>SNANTYTAEEVVESGHRFFGSTSGGIASAVEKAFQSFGLPNGYILGEEGSGAFIGGLTYGEGTLYTKNAGDHKTFWQGPSLGWDFGGQGSRVMMLVYNLDDIQHLYGRYAGVAGSAYVIAGVGFNVLKRENIVLVPIRTGIGARLGVNIGYLKLSAAPTW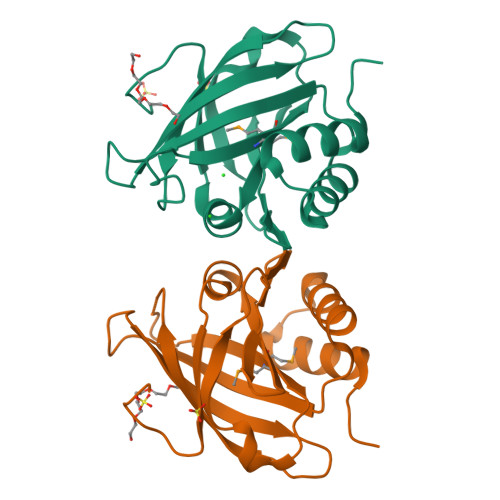NPF[2x]>[2x]GSDNLSRHDMLAWINESLQLNLTKIEQLCSGAAYCQFMDMLFPGSIALKKVKFQAKLEHEYIQNFKILQAGFKRMGVDKIIPVDKLVKGKFQDNFEFVQW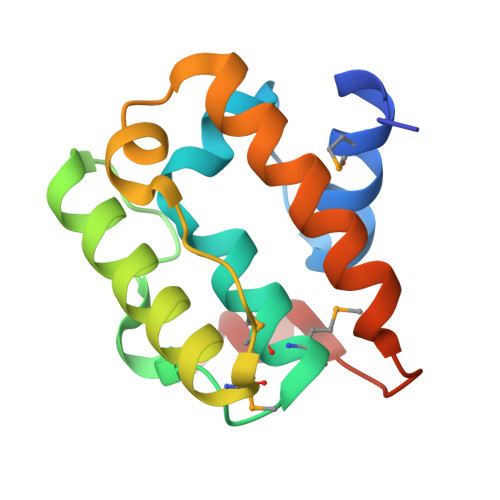FKKFFDANYDGKDYDPVAARQGQ>MHHHHHHSSGRENLYFQGEEEGEDEEELSGTKVSAPYYSSWGTLEYHNAMV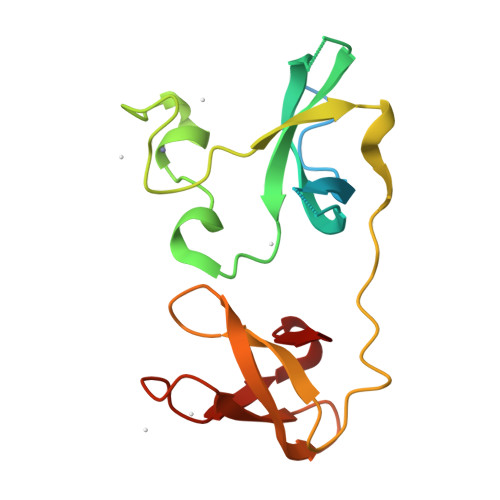VGTEEAEDGSAGVRVLYLYPTHKSLKPCPFFLEGKCRFKENCRFSHGQVVSLDELRPFQDPDLSSLQAGSACLAKHQDGLWHAARITDVDNGYYTVKFDSLLLREAVVEGDGILPP[4x]>MQLLTNHLGYERLGAKQAILQAQPTLALHHADIICCQSGQSIMQLPLQACGPVAQWHIGDTYSIDFTALNICGDYRIRVGDTESASFCVAEGLLMQNTFSDVLHYFKSQRCSGIYECADKKVPLFGTNETVDVHGGWYDASGDVSKYFSHLSYGNYLNPQQTPMVVWNMLTAYEVLEDEESIADFTRVRLVEEALYGADFLLRMQHPQGYFYMTVFDKWSKSTEQREVCAFSTQDGHKSADYQAGFRQGAGVAIAALAAASRLSNLASTSRIPQCGDIKADTYLEAAKKGYWHLKEMNHQYLDNGKENIIDEYCALLASVELYRSTQENNFLAEARMWADKLMARQMSDHNFAHYWAANDDGSRPY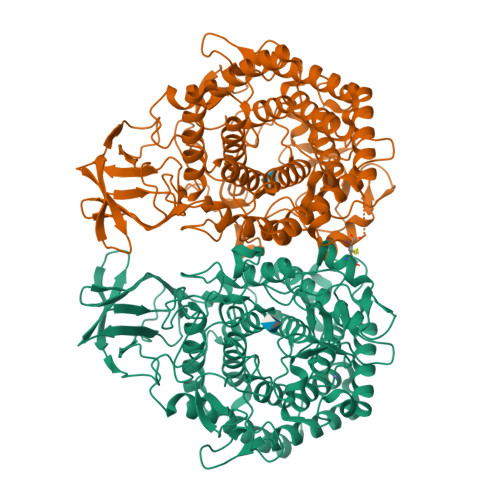FHAAEAGLPAIALMQYLQIETHAQRAEQCQSVLLNALNFELSITHEVNNPFGYPRQYTKAVNGDKQSAFFMPHDNETGYWWQGENARIASLITMAYMAQNTINDNEIKSQLMIYAHRLTDWILGLNPFDMCMLDGHGRNNPDYLPELGFSNAKGGVCNGITSGFENEQGIAFKPEKQKDDMLQNWRWGEQWIPHGAWYLLAITMQFKERNHVLEHHHHHH[2x]> MA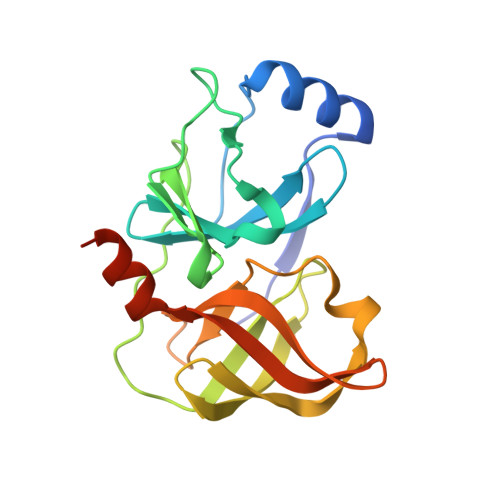PITAYSQQTRGLLGCIITSLTGRDKNQVEGEVQVVSTATQSFLATCVNGVCWTVYHGAGSKTLAGPKGPITQMYTNVDQDLVGWQAPPGARSLTPCTCGSSDLYLVTRHADVIPVRRRGDSRGSLLSPRPVSYLKGSSGGPLLCPSGHAVGIFRAAVCTRGVAKAVDFVPVESMETTMRSGSHHHHHH> MVELTEIKDDVVQLDEPQFSRNQAIVEEKASATNNDVVDDEDDSD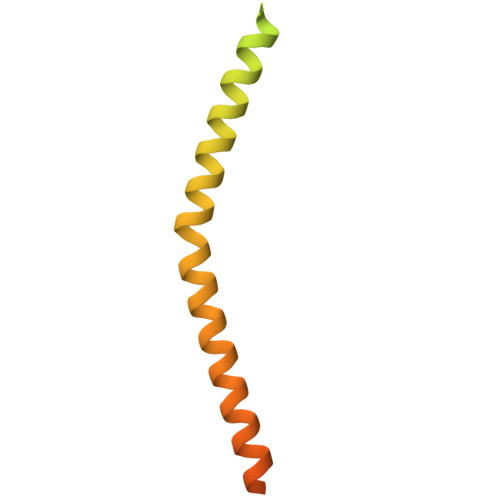SDFEDEFDENETLLDRIVALKDIVPPGKRQTISNFFGFTSSFVRNAFTKSGNLAWTLTTTALLLGVPLSLSILAEQQLIEMEKTFDLQSDANNILAQGEKDAAATANGGHHHHHHHH>[4x]TNMSIKEQRESLPVFQFRDQIIQAVKDNQILIVVGETGSGKTTQVTQYLAEAGFTKYGMIGCTQPRRVAAVSVAKRVAEEVGCQLGQEVGYTIRFEDVTSPATKIKYMTDGMLQREILMDPDLKRYSVIMLDEAHERTIATDVLFALLKKTVKRRPDLKVIVTSATLDAEKFSEYFNSCPIFTIPGRTFPVEILYSREPEPDYL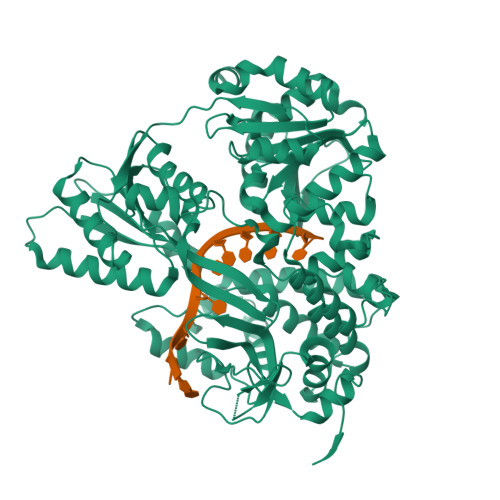EAALTTVMQIHLTEPPGDILVFLTGQEEIDTACEILYERMKALGPSVPELIILPIYSALPSEMQSRIFEPAPPGSRKVVIATNIAETSITIDYIYYVVDPGFVKQNAYDPKLGMDSLVVTPISQAQANQRAGRAGRTGPGKCFRLYTEAAYQSEMLPTTIPDIQRQNLANTILLLKAMGINDLLRFDFMDPPPVNTMLTALEELYALGALDDEGLLTRLGRKMADFPMEPSLSKVLIASVDKGCSDEMVTIVSMLNLQQIFYRPKDKQQQADQKKAKFHDPTGDHLTLLNVYNAWKNSGYSNAWCFENYIQARAMRRARDVRQQIVKIMERHRHPIISCGRDTDKIRQALCAGFFRNTARKDPQEGYKTLTEGTPVYLHPSSALFGKQAEWVLYHELVLTTKEYMHFTTAIEPKWLVEAAPTFFKLAPTDRLSKRKKAERIQPLYNKYEGEDGWRLSAQRRAARPGGGGGTWG>[2x]DKATIPSESPFAAAEVADGAIVVDIAKMKYETPELHVKVGDTVTWINREAMPHNVHFVAGVLGEAALKGPMMKKEQAYSLTFTEAGTYDYHCTPHPFMRGKVVVE;>QDAPEAETQAQETQGQAAARAAAADLAAGQDDEPRILEAPAPDARRVYVNDPAHFAAVTQQFVIDGEAGRVIGMIDGGFLPNPVVADDGSFIAHASTVFSRIARGERTDYVEVFDPVTLLPTADIELPDAPRFLVGTYPWMTSLTPDGKTLLFYQFSPAPAVGVVDLEGKAFKRMLDVPDCYHIFPTAPDTFFMHCRDGSLAKVAFGTEGTPEITHTEVFHPEDEFLINHPAYSQKAGRLVWPTYTGKIHQIDLSSGDAKFLPAVEALTEAERADGWRPGGWQQVAYHRALDRIYLLVDQRDEWRHKTASRFVVVLDAKTGERLAKFEMGHEIDSINVSQDEKPLLYALSTGDKTLYIHDAESGEELRSVNQLGHGP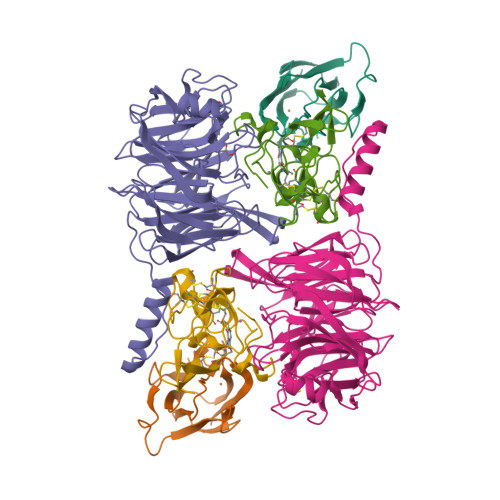QVITTADMG[2x];>ADAPAGTDPRAKWVPQDNDIQACDYWRHCSIDGNICDCSGGSLTNCPPGTKLATASWVASCYNPTDGQSYLIAYRDCCGYNVSGRCPCLNTEGELPVYRPEFANDIIWCFGAEDDAMTYHCTISPIVGKAS[2x]> MFIYYKRTKQGSTEQWFVIGGKRIYLPTMTYVNEANDLIKRYGGNTNVTTYNHDNFGLKMMEAALPQVKV

Endolysins are hydrolytic enzymes that specifically recognize the host cell-wall and cleave the peptidoglycan to digest the bacterial cell-wall for release of phage progeny during the lytic cycle, which is why they hold promise for the treatment of multidrug-resistant bacterial infections as an alternative to antibiotics. LysIME-EF1, an endolysin isolated from E. faecalis phage possesses a highly efficient lytic activity to multidrug resistance E. faecalis. PSI-BLAST search predicted that LysIME-EF1 consists of an N-terminal catalytic CHAP (cysteine, histidine-dependent amidohydrolases/peptidases) domain and a C-terminal CBD (cell-wall binding domain). Our finding provides structural and functional evidence that LysIME-EF1 belongs to a unique two-component multimeric endolysin encoded by a single gene.

Following extensive crystallization trials, we obtained crystals that diffracted well in the space group I422, with cell parameters a = b = 59.88 Å, c = 87.01 Å, α = β = γ = 90.00°. Ultimately, the dataset diffracted in the space group I422 was proved to be LysIME-EF1 CBD and the structure was solved by molecular replacement method at 1.75 Å resolution using the CBD from WT LysIME-EF1 as a search model. There was one molecule in an asymmetric unit. The CBD comprises a four-stranded β-sheet capped on each side by one α-helix. Crystallographic symmetry analysis suggested that LysIME-EF1 CBD forms a stable homotetramer. The oligomeric interface contains 1318.9 Å2 of the buried surface area, accounting for 28.25% of the monomer surface area calculated by PISA. The LysIME-EF1 CBD was cloned into pET 21a(+) with an N-terminal His tag and the purified LysIME-EF1 CBD was subjected to size-exclusion chromatography and the elution profile is 17.7 ml in a Superdex 200 column (GE Healthcare) with an estimated ~32 kDa, supporting that LysIME-EF1 CBD forms a stable tetramer in solution. Detailed analysis shows that the tetramerization is mainly mediated by extensive hydrogen bonds and hydrophobic interactions. In addition, a sizeable hydrophobic interface is formed by the neighboring protomers, where the residues M227, M228, A230, A231, L232 of α2 helix from one protomer pack against hydrophobic patches 183WFVIGG188 and 191IYLP194 of the other protomer. Differing from that of LysIME-EF1 CBD, the elution profile of the LysIME-EF1 CBD F184R&Y218A is 18.7 ml, confirming that the residues F184 and Y218 are essential for maintaining the oligomeric tetramerization of LysIME-EF1.>[4x]MSLAPRPRILICEDDPDIARLLNLMLEKGGFDSDMVHSAAQALEQVARRPYAA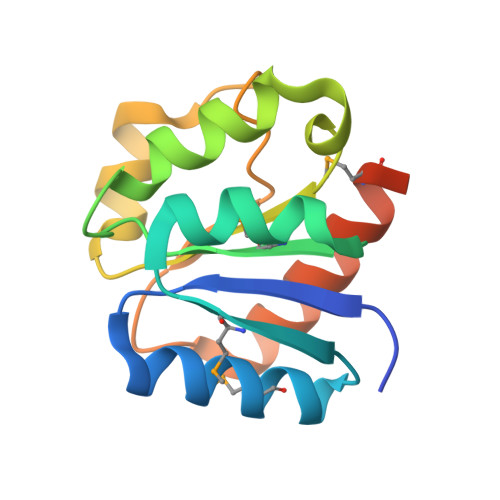MTVDLNLPDQDGVSLIRALRRDSRTRDLAIVVVSANAREGELEFNSQPLAVSTWLEKPIDENLLILSLHRAIDNMAEGKEGHHHHHH>STILVIHGPNLNLLGKREPEVYGHLTLDNINRQLIAQAEQASITLDTFQSNWEGAIVDRIHQAQTEGVKLIIINPAALTHTSVALRDALLGVAIPFIEVHLSNVHAREAFRHHSYLSDKAIGVICGLGAKGYSFALDYAIEKIQP[11x];> MSS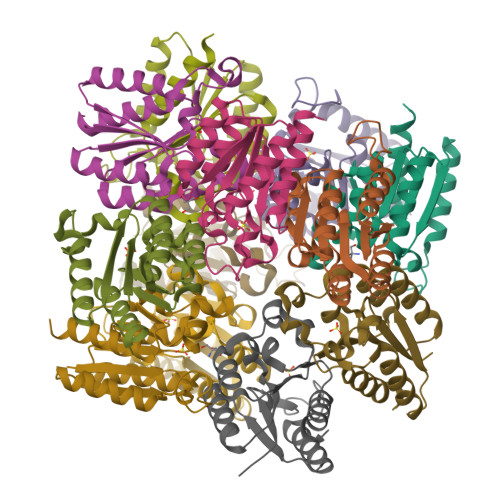TILVIHGPNLNLLGKREPEVYGHLTLDNINRQLIAQAEQASITLDTFQSNWEGAIVDRIHQAQTEGVKLIIINPAALTHTSVALRDALLGVAIPFIEVHLSNVHAREAFRHHSYLSDKAIGVICGLGAKGYSFALDYAIEKIQP>GITGTWYNQLGSTFIVTAGADGALTGTYESAVGNAESRYVLTGRYDSAPATDGSGTALGWTVAWKNNYRNAHSATTWSGQYVGGAEARINTQWLLTSGTTEANAWKSTLVGHDT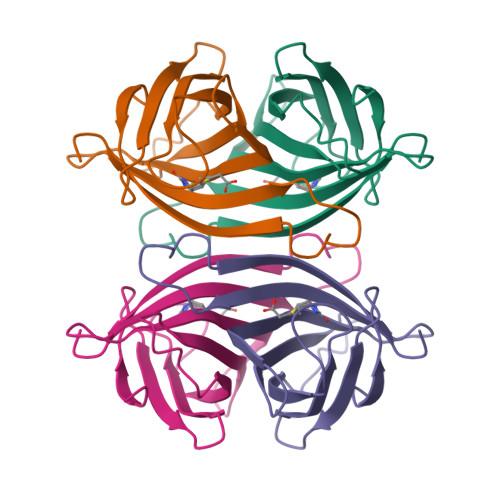FTKVK[4x]N-[(3S,4R,5R,6S)-4,5,6-trihydroxyazepan-3-yl]butanamide 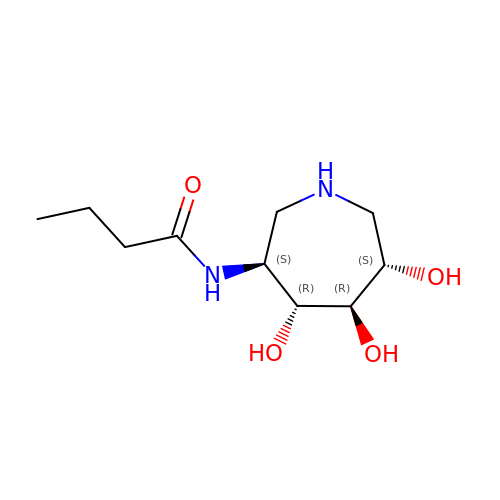| C10 H20 N2 O4 | SWEITPYHDWSHKI-AKEJEFCPSA-N> KEATWVTDKPLTLKIHMHFRDKWVWDENWPVAKESFRLTNVKLQSVANKAATNSQEQFNLMMASGDLPDVVGGDNLKDKFIQYGQEGAFVPLNKLIDQYAPHIKAFFKSHPEVERAIKAPDGNIYFIPYVPDGVVARGYFIREDWLKKLNLKPPQNIDELYTVLKAFKEKDPNGNGKADEVPFIDRHPDEVFRLVNFWGARSSGSDNYMDFYIDNGRVKHPWAETAFRDGMKHVAQWYKEGLIDKEIFTRKAKAREQMFGGNLGGFTHDWFASTMTFNEGLAKTVPGFKLIPIAPPTNSKGQRWEEDSRQKVRPDGWAITVKNKNPVETIKFFDFYFSRPGRDISNFGVPGVTYDIK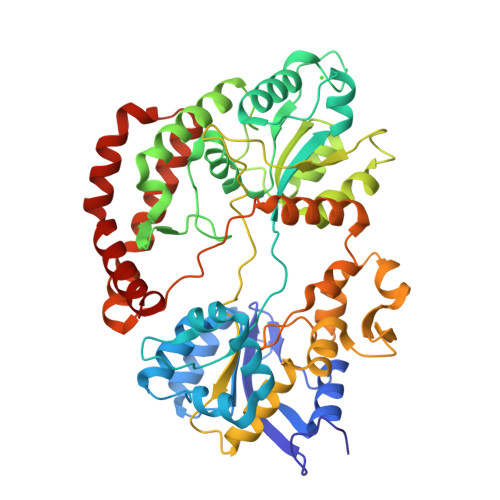NGKAVFKDSVLKSPQPVNNQLYDMGAQIPIGFWQDYDYERQWTTPEAQAGIDMYVKGKYVMPGFEGVNMTREERAIYDKYWADVRTYMYEMGQAWVMGTKDVDKTWDEYQRQLKLRGLYQVLQMMQQAYDRQYKN>[4x]MKSWAAAVALMVGILSPHAAAAPPANPVQRDMLQVLEARQSGPTCNTPSNRACWTNGFDINTDYEVSTPNTGRTVAYQLTLTEKENWIGPDGVLKNVVMLVNDKIIGPTIRANWGDNIEVTVINNLKTNGTSMHWHGLRQLGNVFNDGANGVTECPIPPKGGRKTYKFRATQYGTSWYHSHFSAQYGNGVVGTIQI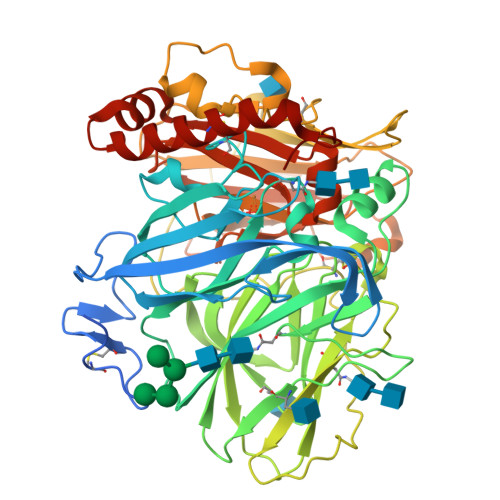DGPASLPYDIDLGVFPLMDYYYRSADELVHFTQSNGAPPSDNVLFNGTARHPETGAGQWYNVTLTPGKRHRLRIINTSTDNHFQVSLVGHNMTVIATDMVPVNAFTVSSLFLAVGQRYDVTIDANSPVGNYWFNVTFGDGLCGSSNNKFPAAIFRYQGAPATLPTDQGLPVPNHMCLDNLNLTPVVTRSAPVNNFVKRPSNTLGVTLDIGGTPLFVWKVNGSAINVDWGKPILDYVMSGNTSYPVSDNIVQVDAVDQWTYWLIENDPTNPIVSLPHPMHLHGHDFLVLGRSPDELPSAGVRHIFDPAKDLPRLKGNNPVRRDVTMLPAGGWLLLAFKTDNPGAWLFHCHIAWHVSGGLSVDFLERPNDLRTQLNSNAKRADRDDFNRVCREWNAYWPTNPFPKIDSGL>[2x]MSAPTPLAEASQIPTIPALSPLTAKQSKGNFFSSNPISSFVVDTYKQLHSHRQSLELVNPGTVENLNKEVSRDVFLSQYFFTGLRADLNKAFSMNPAFQTSHTFSIGSQALPKYAFSALFANDNLFAQGNIDNDLSVSGRLNYGWDKKNISKVNLQISDGQPTMCQLEQDYQASDFSVNVKTLNPSFSEKGEFTGVAVASFLQSVTPQLALGLETLYSRTDGSAPG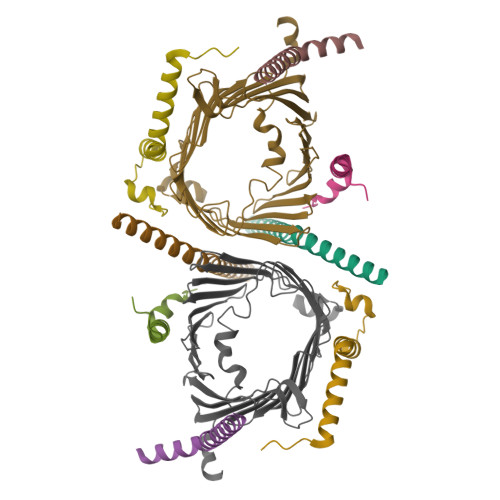DAGVSYLTRYVSKKQDWIFSGQLQANGALIASLWRKVAQNVEAGIETTLQAGMVPITDPLMGTPIGIQPTVEGSTTIGAKYEYRQSVYRGTLDSNGKVACFLERKVLPTLSVLFCGEIDHFKNDTKIGCGLQFETAGNQELLMLQQGLDADGNPLQALPQL;>[2x]MVELTEIKDDVVQLDEPQFSRNQAIVEEKASATNNDVVDDEDDSDSDFEDEFDENETLLDRIVALKDIVPPGKRQTISNFFGFTSSFVRNAFTKSGNLAWTLTTTALLLGVPLSLSILAEQQLIEMEKTFDLQSDANNILAQGEKDAAATANRTLQVDGSPGHHHHHHHHHH;>[2x]MFGLPQQEVSEEEKRAHQEQTEKTLKQAAYVAAFLWVSPMIWHLVKKQWK;>[2x]MDGMFAMPGAAAGAASPQQPKSRFQAFKESPLYTIALNGAFFVAGVAFIQSPLMDMLAPQL;>MSFLPSFILSDESKERISKILTLTHNVAHYGWIPFVLYLGWAHTSNRPNFLNLLSPLPSV[2x]>MQEIALTPQPAHLTVKDGRFEFGNQLKAKVTPYQGDSIRMVFESFKKELQEATGIKVSSTQKEAKARIILDLNPQLPAEAYKLNVSKKQVRIEASRPAGFYYALQTLKQLMPRNVMAGVATSDHSQWSLPSVEIEDAPRFEWRGFMLDEGRHFFGKDEIKRVIDMMAIYKMNRFHWHLTEDQGWRIEIKKYPKLTETGAWRNSKVLAYGDVKPDGERYGGFYTQKDIKEIVAYAKKKFIEIIPEIDIPGHSQAAVAAYPEFLACDPRDKHEVWLQQGIST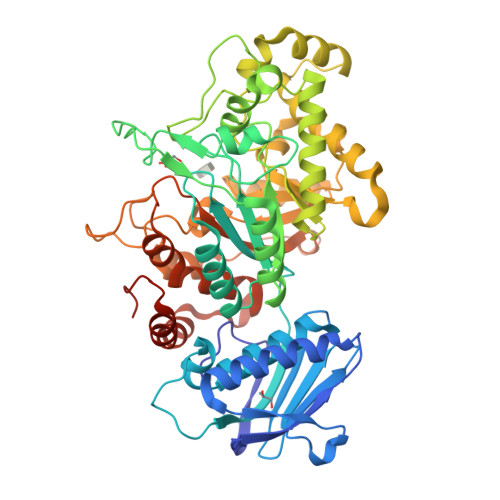DVINVANPKAMQFAKEVIDELTELFPFNYIHLGGDECPTRKWQKNDECKKLLSEIGSSNFRDLQIYFYKQLKDYIATKPADQQRQLIFWNEVLHGNTSILGNDITIMAWIGANAAAKQAAKQGMNTILSPQIPYYINRKQSKLPTEPMSQGHGTETVEAVYNYQPLKDVDAALQPYYKGVQANFWTEWVTEPSVLEYLMLPRLAAVAEAGWTPQEKRNYEDFKERIRKDAELYDLKGWNYGKHIMKLEHHHHHH[2x]E-64 is an irreversible cysteine protease inhibitor prominently used in chemical biology and drug discovery. Here we uncover a nonribosomal peptide synthetase-independent biosynthetic pathway for E-64, which is widely conserved in fungi. The pathway starts with epoxidation of fumaric acid to the warhead (2S,3S)-trans-epoxysuccinic acid with an Fe(II)/α-ketoglutarate-dependent oxygenase, followed by successive condensation with an l-amino acid by an adenosine triphosphate grasp enzyme and with an amine by the fungal example of amide bond synthetase. Both amide bond-forming enzymes display notable biocatalytic potential, including scalability, stereoselectivity toward the warhead and broader substrate scopes in forming the amide bonds.

Therefore, the first amide bond between (2S,3S)-t-ES and l-Ile is catalyzed by Cp1B, while formation of the second amide bond between 14 and putrescine is catalyzed by Cp1D. Cp1B is also enantiospecific for (2S,3S)-t-ES and steady-state kinetics showed that Cp1B phosphorylated (2S,3S)-t-ES with kcat/KM (apparent) of 48.0 mM−1 min−1. The X-ray crystal structure of Cp1B complexed with adenosine and 2-morpholinoethanesulfonic acid (MES) was determined to 2.7-Å resolution. The ATP-binding site in Cp1B where adenosine resides is partially covered by the lid domain with the P-loop and the A-loop from domain A52, indicating that the Cp1B structure is in the closed form. This unexpected closed form without a substrate or product could result from the binding of the buffer MES molecule in the active site. The morpholine moiety of MES is found to be housed in the hydrophobic pocket with F175, V228, V477 and I488. Docking simulation of (2S,3S)-t-ES-l-Phe with Cp1B showed that the side chain of l-Phe can also be housed in the same hydrophobic pocket, suggesting that the MES-binding site could be where the side chain of the l-amino acid binds. Similar to the ATP-binding site of hGSH synthetases, the adenosine in the Cp1B structure is sandwiched between the strands of two antiparallel β-sheets and is surrounded by the conserved residues R139, D141, E163 and N165, which are likely involved in generation of the acyl-phosphate intermediate. Individual substitutions of each residue to alanine either abolished or significantly attenuated enzymatic activity of Cp1B. Hence, although annotated as a HP, our biochemical and structural characterization demonstrated that Cp1B is the biochemically validated example of an ATP-grasp enzyme in fungal natural product biosynthesis.

> HHHHHHSSGLVPRGSMKIPAPQQLQQLHVSLDGGHYEPVTTFDPAKATYLQDQEALQENLLRLCSVNGWHKSSRAACSPRPVLVSSEHQRRWRELHEALVLAITDIVERWLTDPEARFPERMPLEPEEEDLLRWIDEQVPHNLPQYRDCRGSWRPDFLVEEENSEDGSGPVENFRISEINARFSFNGFMFATCGQQAIHDMGICDNGNGLVGATDPAKILKGLLRLFQPGLPLHLLKGDEAGVDIHMLVDFLDRYLGITPRFIMPADLRLLHEPQAKGGYKLCCVVKNPDSCDPATLIYHDGDILEEIHQVGLELHQREIRALEPEMLRQISLRCFNDMRTILLVHDKRMLGIVRQELENLVARNVLTLSQAKILDKGIPETILPGSLDLDQAIARCKEMPELKDEYILKPIRSGKGDGIVFGEDLNSEEWISRLEGLRSAQLIPGGGTCIVQRKVKQLLYDVVLRPTGVKTRYPLIGTYHSINGEFLGVGVWRSSPDRICAISHGGAWTVSVMRDE The human mannose receptor expressed on macrophages and hepatic endothelial cells scavenges released lysosomal enzymes, glycopeptide fragments of collagen, and pathogenic microorganisms and thus reduces damage following tissue injury. The receptor binds mannose, fucose, or N-acetylglucosamine (GlcNAc) residues on these targets. C-type carbohydrate-recognition domain 4 (CRD4) of the receptor contains the site for Ca2+-dependent interaction with sugars. The mechanisms of binding to monosaccharides and oligosaccharide substructures present in many of these ligands were examined in multiple crystal structures of CRD4.

The binding of α-methyl mannose to CRD4 is revealed by four independent copies of this complex observed in three different crystal forms: two copies of the CRD in form αMeMan/1 and one copy of the CRD in αMeMan/2 and αMeMan/3. Each structure shows the same orientation of the bound sugar. Binding of mannose residues to CRD4 results primarily from interaction of the equatorial 3- and 4-OH groups with a conserved principal Ca2+ common to almost all sugar-binding C-type CRDs. As in other C-type CRDs, the main determinants of monosaccharide binding to CRD4 are a conserved principal Ca2+ and four of the five amino acid residues that surround it. In addition to the Ca2+ ligands, the side chain of Tyr729 makes van der Waals contacts with the bound sugar. The position of the aromatic ring of Tyr729 is established in part by interactions with the side chain of Gln730. In some of the crystal forms, the conformation of the side chain of Ile749 produces an additional contact with the bound sugar. For example, while there is a single conformation of the side chain of Ile749 in the αMeMan/3 crystals, there are multiple conformations in the αMeMan/1 crystals. In the αMeMan/1 crystals, the electron density map shows multiple conformations for Ser671 and Glu677. These side chains, as well as the Ca2+, have been modeled at 50% occupancy, with one of the partially occupied chain conformations binding to the Ca2+.

>[2x]ACPEDWGASSRTSLCFKLYAKGKHEKKTWFESRDFCRALGGDLASINNKEEQQTIWRLITASGSYHKLFWLGLTYGSPSEGFTWSDGSPVSYENWAYGEPNNYQNVEYCGELKGDPTMSWNDINCEHLNNWICQI>MASKPQPIAAANWKCNGSQQSLSELIDLFNSTSINHDVQCVVAPTFLHIPMTKARLTNPKFQIAAQNAITRSGAFTGEVSLQILKDYGISWVVLGHSERRAYYGETNEIVADKVAAAVASGFHVIVCVGETNEEREAGRTAAVVLTQLAAVAQKLSKEAWSRVVIAYEPVWAIGTGKVATPQQAQEVHELLRRWVRSKLGTDIAAQLRILYGGSVTAKNARTLYQMRDINGFLVGGASLKPEFVEIIEATK[4x]

Take for example the glycolytic enzyme triosephosphate isomerase (TIM) from two evolutionarily related pathogenic parasites, Trypanosoma brucei and T. cruzi. Many of the proteins of these parasites have a high degree of sequence identity; in the case of the two trypanosomal TIMs it is 73.9%, with a sequence similarity of 92.4%. Both enzymes are homodimers whose three dimensional structures superpose with an RMS of 0.96 Å and both have an identical catalytic site in each monomer formed by residues K13, H95 and E167 (based on the numbering for the sequence of TIM from T. brucei (TbTIM)). Of particular relevance to this work is their remarkably different susceptibility to sulfhydryl reagents like methylmethane thiosulfonate (MMTS): the enzyme from T. cruzi is 70 times more sensitive than the enzyme from T. brucei. The initial site of action of the thiol reagent in both enzymes is their only interface cysteine (Cys), which is at position 14 or 15 of TbTIM and TIM from T. cruzi (TcTIM), respectively; it is surrounded by residues of loop 3 of the other subunit.

We therefore designed a chimera of TcTIM with regions 1 and 4 of TbTIM (TcTIM 2,3, 5–8). This chimera and WT TbTIM exhibited almost identical inactivation profiles at low and high concentrations of MMTS. Taken together, the data with chimeras TcTIM 1 and TcTIM 2,3, 5–8 it may be concluded that, at most, the 13 different amino acids in region 1 of the two WT enzymes account for their different susceptibilities to MMTS at concentrations higher than 50 µM. In order to check for the absence of major conformational differences due to the sequence perturbations on the chimeras, we solved the crystal structure at 1.65 Å resolution of chimera TcTIM 2,3, 5–8. The analysis of the structure shows that the chimera can be superposed on the crystal structures of TcTIM and TbTIM with a RMSD of 0.385 and 0.437 Å respectively, with a minor displacement on the loop of region 1. A displacement in region 6 is also observed, which corresponds to the amino acids of the flexible loop involved in enzyme catalysis. Thus, it can be suggested that the disparities in susceptibility to thiol reactive agents between the different proteins produced by changes in regions 1 and 4 are due to the effect of their side chains and not to any major rearrangement of the main chain. When the pKa of the thiol group for Cys 14/15 of the wild type enzymes and the chimerical enzyme TcTIM 2,3, 5–8 were determined anew, under the same conditions, the values turned out to be 9.27, 10.53 and 10.61 for TcTIM, TbTIM and TcTIM 2,3, 5–8, respectively. Altogether, the data show that the relevant residues of regions 1 and 4 modulate the reactivity of the interface Cys through long-range interactions and that the interface residues do not play a role in the susceptibility to MMTS.> GMQVEGLSINLATIREQCGFAEAVDICLKHGITAIAPWRDQVAAIGLGEAGRIVRANGLKLTGLCRGGFFPAPDASGREKAIDDNRRAVDEAAELGADCLVLVAGGLPGGSKNIDAARRMVVEGIAAVLPHARAAGVPLAIEPLHPMYAADRACVNTLGQALDICETLGPGVGVAIDVYHVWWDPDLANQIARAGKMKAILAHHICDWLVPTKDMLTDRGMMGDGVIDLKG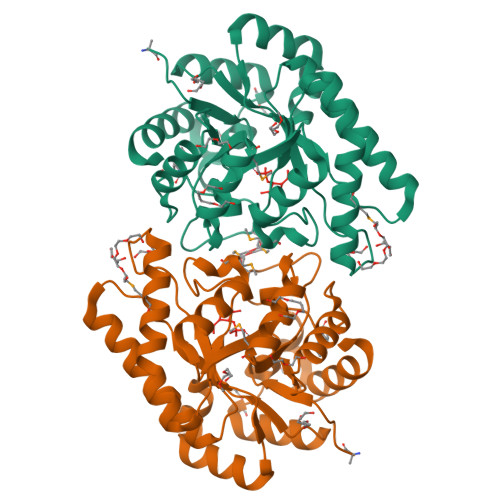IRRRIEAAGFHGAQEVEIFSADNWWKRPADEVIATCVERYRNCC> GAGCAACUUAGGA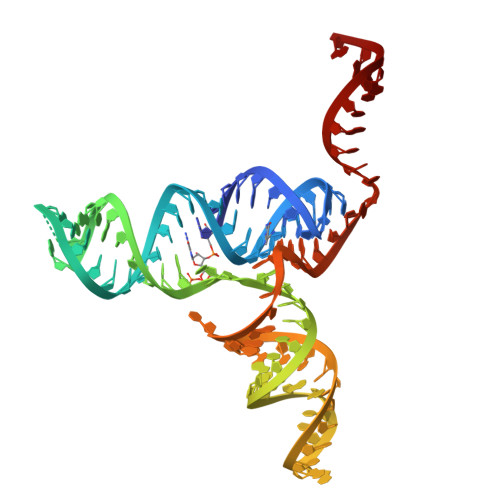UUUUAGGCUCCCCGGCGUGUCUCGAACCAUGCCGGGCCAAACCCAUAGGGCUGGCGGUCCCUGUGCGGUCGAAAUUCAUCCGCCGGAG> MGHHHHHHGEFKALTRRLQVEPRLLSKQMAGCLEDCTRQAPESPWEEQLARLLQEAPGKLSLDVEQAPSGQHSQAQLSGQQQRLLAFFKCCLLTDQLPLAHHLLVVHHGQRQKRKLLTLDMYNAVMLGWARQGAFKELVYVLFMVKDAGLTPDLLSYAAALQCMGRQDQDAGTIERCLEQMSQEGLKLQALFTAVLLSEEDRATVLKAVHKVKPTFSLPPQLPPPVNTSKLLRDVYAKDGRVSYPKLHLPLKTLQCLFEKQLHMELASRVCVVSVEKPTLPSKEVKHARKTLKTLRDQWEKALCRALRETKNRLEREVYEGRFSLYPFLCLLDEREVVRMLLQVLQALPAQGESFTTLARELSARTFSRHVVQRQRVSGQVQALQNHYRKYLCLLASDAEVPEPCLPRQYWEALGAPEALREQPWPLPVQMELGKLLAEMLVQATQMPCSLDKPHRSSRLVPVLYHVYSFRNVQQIGILKPHPAYVQLLEKAAEPTLTFEAVDVPMLCPPLPWTS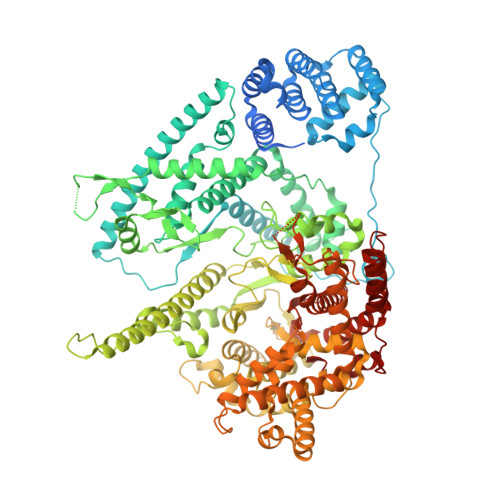PHSGAFLLSPTKLMRTVEGATQHQELLETCPPTALHGALDALTQLGNCAWRVNGRVLDLVLQLFQAKGCPQLGVPAPPSEAPQPPEAHLPHSAAPARKAELRRELAHCQKVAREMHSLRAEALYRLSLAQHLRDRVFWLPHNMDFRGRTYPCPPHFNHLGSDVARALLEFAQGRPLGPHGLDWLKIHLVNLTGLKKREPLRKRLAFAEEVMDDILDSADQPLTGRKWWMGAEEPWQTLACCMEVANAVRASDPAAYVSHLPVHQDGSCNGLQHYAALGRDSVGAASVNLEPSDVPQDVYSGVAAQVEVFRRQDAQRGMRVAQVLEGFITRKVVKQTVMTVVYGVTRYGGRLQIEKRLRELSDFPQEFVWEASHYLVRQVFKSLQEMFSGTRAIQHWLTESARLISHMGSVVEWVTPLGVPVIQPYRLDSKVKQIGGGIQSITYTHNGDISRKPNTRKQKNGFPPNFIHSLDSSHMMLTALHCYRKGLTFVSVHDCYWTHAADVSVMNQVCREQFVRLHSEPILQDLSRFLVKRFCSEPQKILEASQLKETLQAVPKPGAFDLEQVKRSTYFFS> KGKSEVVEQNHTLILGWSDKLGSLLNQLAIANESLGGGTIAVMAERDKEDMELDIGKMEFDFKGTSVICRSGSPLILADLKKVSVSKARTIIVLAEDGNADQSDARALRTVLSLTGVKEGLRGHIVVEMSDLDNEVLVKLVGGDLVETVVAHDVIGRLMIQCARQPGLAQIWEDILGFENCEFYIKRWPQLD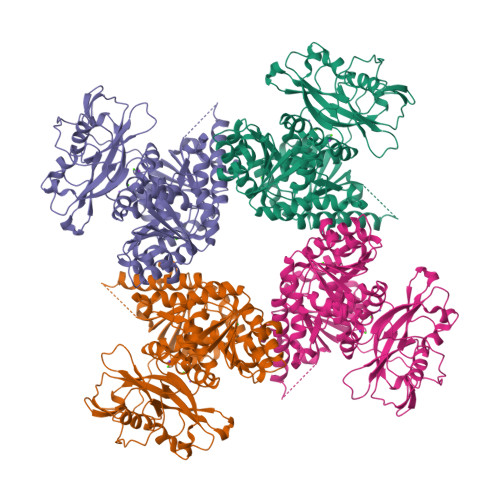GMLFEDVLISFPAAIPCGIKVASYGGKIILNPDDSYVLQEGDEVLVIAEDDDTYAPAPLPMVRRGSLPKDFVYPKSPERILFCGWRRDMEDMITVLDASLAPDSELWMFNDVPEKEREKKLIDGGLDISRLENISLVNREGNAVIRRHLESLPLESFDSILILADESVEDSAIQADSRSLATLLLIRDIQARRLPYVAMASQTQGGNFSKGSWIGEMKQASDKTVIISEILDPRTKNLLSMSKISDYVLSNELVSMALAMVAEDRQINDVLEELFAEEGNEMHIRQADIYLREGEEMSFYEIMLRARQRREILIGYRLANAERAVINPPAKTGRRKWSLKDVFVVITEKE>VERMYDVTPPGVVMGLAWTAMGGSTLFVETSLRRPQDKDAKGDKDGSLEVTGQLGEVMKESARIAYTFARAFLMQHAPANDYLVTSHIHLHVPEGATPKDGPS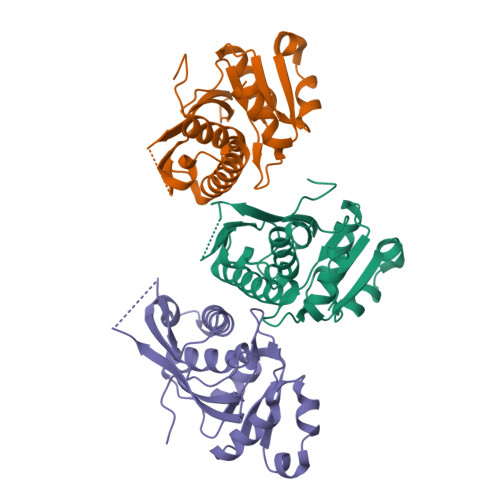AGCTIVTALLSLAMGRPVRQNLAMTGEVSLTGKILPVGGIKEKTIAAKRAGVTCIVLPAENKKDFYDLAAFITEGLEVHFVEHYREIFDIAFPDEQAEALAVER[6x]> DDNEDGFIADSDIISRSDFPKSWLWLTKDLTEEPNSQGISSKTMSFYLRDSITTWVVLAVSFTPTKGICVAEPYEIRVMKVFFIDLQMPYSVVKNEQVEIRAILHNYVNEDIYVRVELLYNPAFCSASTKGQRYRQQFPIKALSSRAVPFVIVPLEQGLHDVEIKASVQEALWSDGVRKKLKVVPEGVQKSIVTIVKLDPRAKGVGGTQLEVIKARKLDDRVPDTEIETKIIIQGDPVAQIIENSIDG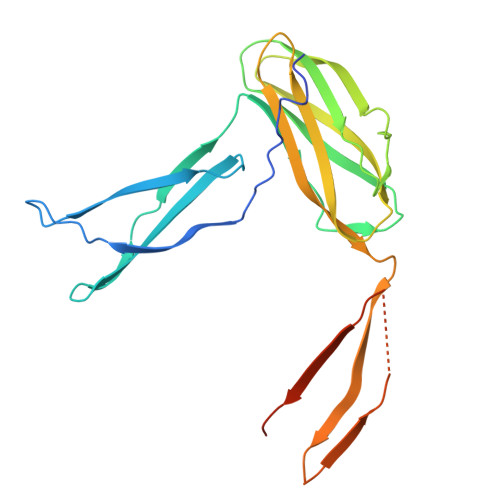SKLN Interleukin (IL-), an IL-6 family cytokine, has pivotal roles in autoimmune diseases, fibrotic complications, and solid cancers. IL-11 activates downstream signalling pathways by binding its two cell surface receptors: the IL-11 specific receptor, IL-11Rα, and the signal-transducing receptor, glycoprotein (gp)13013,26. Following the formation of the receptor complex, the Janus kinase (JAK)/signal transducer and activator of stat (STAT) and extracellular signal regulated kinase (ERK)/mitogen-activated protein kinase (MAPK) pathways are primarily activated. IL-11 and IL-6 utilise a homodimer of gp13026,34,35 while other IL-6 family members exploit a heterodimer of gp130 with a second signal-transducing receptor, such as LIF receptor (LIFR), OSM receptor (OSMR), IL-27R/WSX-1 or IL-12 receptor β−2 subunit (IL-12Rβ2).

Phage display was subsequently used to identify variants with higher inhibitory potency resulting in IL-11 Mutein, which contains W147A combined with mutations of AB loop residues 58–62, 58AMSAG62 to 58PAIDY62, that were reported to increase affinity to IL-11Rα43. We solved crystal structures of IL-11Δ10/Mutein and IL-11Δ10/W147A at resolutions of 1.8 Å and 1.5 Å, respectively, to understand the structural consequences of the mutations. The structure of IL-11Δ10/W147A is similar to the structure of IL-11Δ10 (RMSD 0.3 Å relative to IL-11Δ1049), indicating that the W147A mutation does not alter the structure. In contrast, the AB loop of IL-11Δ10/Mutein shows significant conformational shifts relative to the WT structure caused by alterations in key contacts between the loop and the four-α-helical bundle (Supplementary Fig. 11Gii; RMSD 1.3 Å relative to IL-11Δ1049). Thus, the 58PAIDY62 mutations alter the position of the AB-loop, shifting the register of key loop-core interactions by three residues, while maintaining the composition of the interacting residues. This register change is due to a shift of the LX(S/T)LP motif that mediates loop-core contacts: In IL-11Δ10 and IL-11Δ10/W147A the motif is 51LDSLP55, while in IL-11Δ10/Mutein the interacting motif is 54LPTLP58. The result is that the bulk of the loop is shifted toward site-III and the N-terminal turn of helix-B is unfolded. We note that this configuration of the C-terminal segment of the AB-loop and N-terminal turn of helix-B resembles the structure of wild-type IL-11Δ10 bound within the hexameric complex. In combination, these results indicate that that both IL-11Δ10/W147A and IL-11Δ10/PAIDY can mediate assembly of the hexameric signalling complex, albeit to differing extents, while formation of site III interactions by IL-11Δ10/Mutein is abrogated, and assembly is stalled at the trimer stage.

> GSPDPRAELDSTVLLTRSLLADTRQLAAQLRDKFPADGDHNLDSLPTLPAIDYALGALQLPGVLTRLRADLLSYLRHVQWLRRAGGSSLKTLEPELGTLQARLDRLLRRLQLLMSRLALPQPPPDPPAPPLAPPSSAAGGIRAAHAILGGLHLTLDWAVRGLLLLKTRL> MGSDKIHHHHHH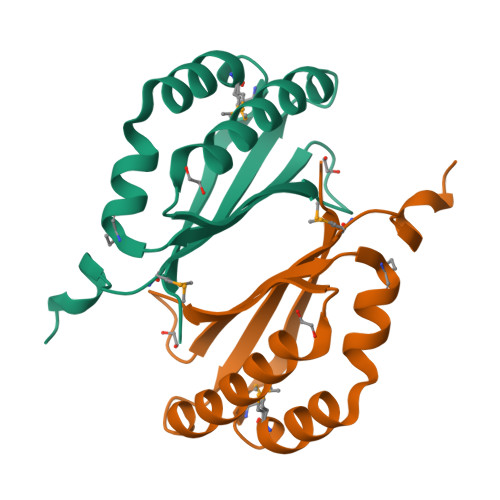ENLYFQGMIGVVATLKVQPAKAAEFEKVFLDLAAKVKANEPGCLVYQLTRSKTEEGVYKVLELYASMDALKHHGGTDYFKAAGAAMGPTMAGAPVIEYLDAVE> MIKNEIKILSDIEHIKKRSGMYIGSSANETHERFMFGKWESVQYVPGLVKLIDEIIDNSVDEGIRTKFKFANKINVTIKNNQVTVEDNGRGIPQAMVKTPTGEEIPGPVAAWTIPKAGGNFGDDKERVTGGMNGVGSSLTNIFSVMFVGETGDGQNNIVVRCSNGMENKSWEDIPGKWKGTRVTFIPDFMSFETNELSQVYLDITLDRLQTLAVVYPDIQFTFNGKKVQGNFKKYARQYDEHAIVQEQENCSIAVGRSPDGFRQLTYVNNIHTKNGGHHIDCAMDDICEDLIPQIKRKFKIDVTKARVKECLTIVMFVRDMKNMRLIRQTKERLTSPFGEIRSHIQLDAKKISRDILNNEAILMPIIEAALARKLAAEKAAETKAAKKASKAKVHKHIKANLCGKDADTTLFLT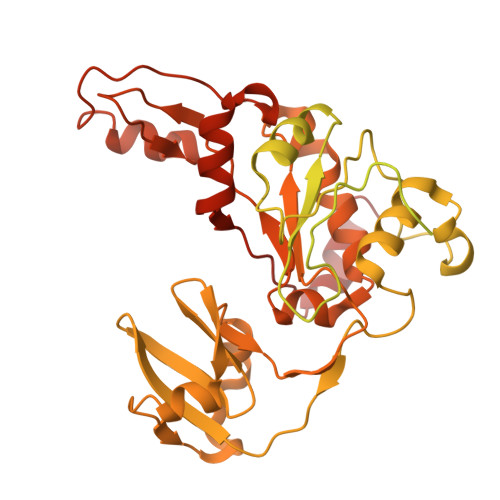EGDSAIGYLIDVRDKELHGGYPLRGKVLNSWGMSYADMLKNKELFDICAITGLVLGEKAFEEKEDGEWFTFELNGDTIIVNENDEVQINGKWITVGELRKNLMKFVKIDSSSVDMKKYKLQNNVRRSIKSSSMNYANVAIMTDADHDGLGSIYPSLLGFFSNWPELFEQGRIRFVKTPVIIAQVGKKQEWFYTVAEYESAKDALPKHSIRYIKGLGSLEKSEYREMIQNPVYDVVKLPENWKELFEMLMGDNADLRKEWMSQHHHHHH Here we identify two Brucella abortus effectors, NyxA and NyxB, that interfere with host protease SENP3, and this facilitates intracellular replication of the pathogen. The translocated Nyx effectors directly interact with SENP3 via a defined acidic patch (identified from the crystal structure of NyxB), preventing nucleolar localisation of SENP3 at late stages of infection. By sequestering SENP3, the effectors promote cytoplasmic accumulation of nucleolar AAA-ATPase NVL and ribosomal protein L5 (RPL5) in effector-enriched structures in the vicinity of replicating bacteria. NyxA/B are two Brucella nucleomodulins impacting the subnuclear localisation of SENP3 and subsequently of other nucleolar proteins such as RPL5 and NVL.

To gain further insight into the function of NyxA and NyxB and their interaction with SENP3, we solved the crystal structure of NyxB at 2.5 Å. The asymmetric unit of the crystal contains 12 monomers of NyxB, but no significant differences were found between them and thus, only the structure of subunit A is described hereafter. The NyxB model encompasses residues 17–134, suggesting that residues 1–16 are flexible. NyxB has a mixed α–β fold with five β strands and six α-helices with a core made of helices α2–α4 and a small curved β-sheet formed by β3–β5. The longest helix α4 interacts with α2 and α6 and is connected to the core via a loop containing two short 310 helices designated α3a and α3b. In particular, a β-hairpin formed by β1 and β2 packs against α5 and anchors α1 to the protein core. Search for structural homologues (DALI server and EMBL fold) did not reveal any significant homology and thus makes of NyxB structure a prototype for this protein family. The association of dimer 1 (chains A and H) buries a total of 530 Å2, while dimer 2 (chains A and J) relies on fewer interactions burying a total of 400 Å2. Analysis of the NyxB surface revealed an acidic pocket delineated by residues Y66, D80 and E82 within an acidic patch consisting of amino acids D72, E73, Y70, Y86 and Y63, residues that are strictly conserved in NyxA. In the context of the dimer, these surfaces are juxtaposed to form an extended concave negatively charged area of around 2000 Å2.

>[12x]MNTQATIDTAAVAPLNFDPNAWHHSQMTTLEAIELSRSGGHPYSSPNVPKGFNTVVGFFFDTYDWYPAAYDDEEGNAMKDRELIQYEDWCAKYARTLGLEVKEVEAPAALKVHGIMALKAYPEALLEIRLIEMP>MEASAGLVAGSHNRNELVVIHGHEEPKPLKNLDGQVCEICGDEIGVTVDGDLFVACNECGFPVCRPCYEYERREGTQQCPQCKTRYKRLKGSPRVEGDEDEEDVDDIEHEFNIDDEQNKHRNVVESILHGKMSYGRGPEDDETPQIPVITGVRSRPVSGEFPIAGALAYGEHMPNA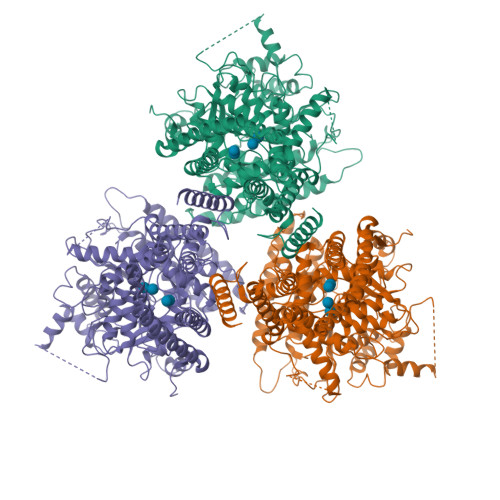SLHKRVHPYPMSETEGAERWDDKKEGGWKERMDDWKMQQGNLGPEADDAYDDMSMLDEARQPLSRKVPIASSKINPYRMVIVARLLILAFFLRYRILNPVHDAIGLWLTSVICEIWFAFSWILDQFPKWFPIDRETYLDRLSLRYEREGEPNMLAPVDIFVSTVDPMKEPPLVTANTVLSILAMDYPVDKISCYISDDGASMLTFESLSETAEFARKWVPFCKKFAIEPRAPEMYFTLKVDYLKDKVQPTFVKERRAMKREYEEFKVRINALVAKAQKVPPEGWIMQDGTPWPGNNTKDHPGMIQVFLGQSGGHDTEGNELPRLVYVSREKRPGFLHHKKAGAMNALVRVSGVLTNAPFMLNLDCDHYINNSKAAREAMCFLMDPQIGRKVCYVQFPQRFDGIDRHDRYANRNTVFFDINMKGLDGIQGPVYVGTGCVFRRQALYGYEPPKGPKRPKMVSCGCCPCFGRRKKDKKYPKNGGNENGPSLEAVEDDKELLMSQMNFEKKFGQSAIFVTSTLMDQGGVPPSSSPAALLKEAIHVISCGYEDKTEWGSELGWIYGSITEDILTGFKMHCRGWRSIYCMPKLPAFKGSAPINLSDRLNQVLRWALGSVEIFFSRHCPAWYGLKGAKLRWLERFAYVNTTIYPFTSLPLLAYCTLPAICLLTDKFIMPPISTFASLFFIALFLSIFATGILELRWSGVSIEEWWRNEQFWVIGGISAHLFAVVQGLLKVLAGIDTNFTVTSKTTDDEEFGELYTFKWTTLLIPPTTVLIINLVGVVAGISDAINNGYQSWGPLFGKLFFSFWVIVHLYPFLKGLMGRQNRTPTIVVIWSVLLASIFSLLWVRIDPFVLKTKGPDTTQCGINC[3x]methyl 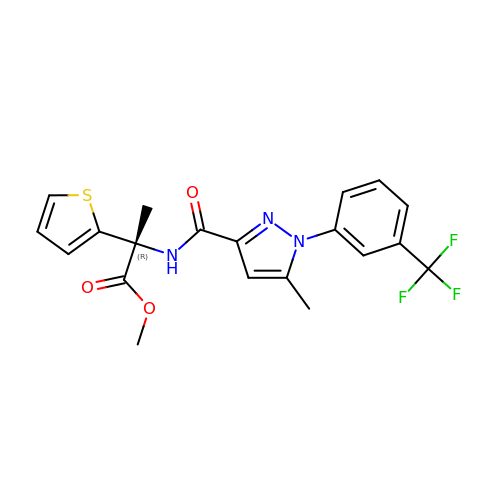(2R)-2-({(1M)-5-methyl-1-[3-(trifluoromethyl)phenyl]-1H-pyrazole-3-carbonyl}amino)-2-(thiophen-2-yl)propanoate | C20 H18 F3 N3 O3 S | XCJKFSDARVULKK-IBGZPJMESA-N5-METHYL-2'-DEOXY-CYTIDINE-5'-MONOPHOSPHATE | C10 H16 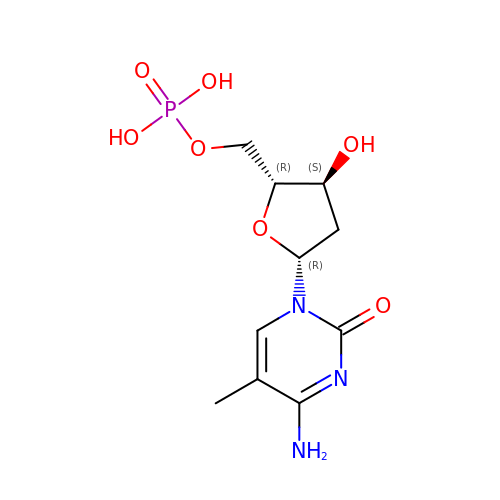N3 O7 P | RGDVNLHBCKWZDA-XLPZGREQSA-N>MAGARRLELGEALALGSGWRHVCHALLYAPDPGMLAGRIPLRYAILMQMRFDGRLGFPGGFVDTQDRSLEDGLNRELREELGEAAAAFRVERTDYRSSHVGSGPRVVAHFYAKRLTLEELLAVEAGATRAKDHGLEVLGLVRVPLYTLRDGVGGLPTFLENSFIGSAREQLLEALQDLGLLQSGSISGLKIPAHH[2x]

A similar cleavage reaction was observed in vitro with other enzymes from diverse organisms, including a snake venom phosphodiesterase (SVP), mammalian ectonucleotide pyrophosphatase/phosphodiesterase 1 (ENPP1), Escherichia coli RppH (EcRppH), and Homo sapiens NudT16 (HsNudT16). In addition, although NudT16 was initially characterized as a nucleolar U8 snoRNA decapping enzyme, it is involved in mRNA decapping and expresses across mouse tissues. Given the versatility in the recognition of substrates with diphosphate bonds, we and others have used some of these Nudix enzymes in vitro for processing ADP-ribosylation to a unique mass tag for site identification by tandem mass spectrometry (MS/MS). In this study, we sought to understand how HsNudT16 binds and hydrolyzes different forms of ADPr using X-ray crystallography.

F36A and F61S mutants were designed to enlarge the mouth of the enzyme with the aim of easing the recognition and processing of the ADPr conjugated to proteins. The crystal structures of mutants F36A and F61S show that the replacement of the phenyl side chain of these residues with a methyl or a hydroxymethyl group, respectively, opens up the mouth of the enzyme. The structural overlap of the HsNudT16-ADPr complex structure with the F36A structure shows that the binding pocket opens up close to the ribose by about 3 Å. The ~9 Å width of the cavity at the Phe36′ to Phe61 increases to 12.6 Å in the F36A mutant. Interestingly, mutation of residue F36A results in a displacement of retention volume from ~10.5 ml (HsNudT16, HsNudT16 H24W and HsNudT16 F61S), which correspond to a molecular weight of 40 kDa, to a retention volume of ~11.2 mL (HsNudT16 F36A and F36A F61S), which correspond to a molecular weight of 27 kDa. This change in retention volume suggests that the lack of phenylalanine at position 36 weakens the dimer, shifting the population to a monomer. In accordance to this shift, analysis of buried surface upon dimerization shows a reduction from about 1320 Å2 in HsNudT16 to about 1210 Å2 in HsNudT16 F36A, where residues 33–36, 50–56 and 120–162 are defined as part of the dimeric interface. Widening the mouth of HsNudT16 at the level of the non-adenosine ribose seems to be deleterious for ADPr hydrolysis activity since the F36A mutant is less active. Crystallization was successful for the H24W, F36A, and F61S mutants and the structures helped rationalized the effects of our single-point mutations. Despite co-crystallization efforts with ADPr, electron density for the substrate could not be seen in the binding site of these mutants.N4-[4-[(6-chloranyl-2-methoxy-acridin-9-yl)amino]butyl]-1,3,5-triazine-2,4,6-triamine 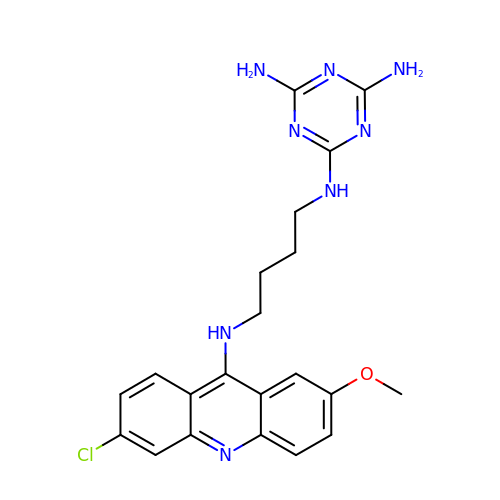| C21 H23 Cl N8 O | YRQBNFDRSZQBNL-UHFFFAOYSA-N9-{hydroxy[(5S,6R)-6-hydroxy-6-{[(1S)-3-{[(3S)-1-hydroxy-2-oxoazepan-3-yl]amino}-1-methyl-3-oxopropyl]oxy}-5-({[(4S)-2-(2-hydroxyphenyl)-4,5-dihydro-1,3-oxazol-4-yl]carbonyl}amino)hexyl]amino}-9-oxononanoic 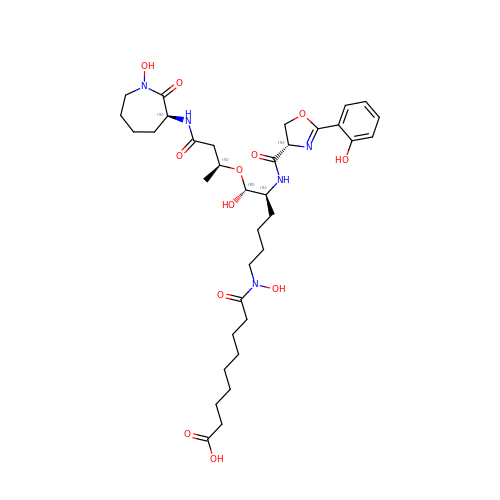acid | C35 H53 N5 O12 | IAYIKQLBDQWIRR-QMSOLXAJSA-N> SNADHHAWHRLLDRALSEQHFQLYFQPVVAARDTHLVLHYKVLSRLLDEQGQTIPA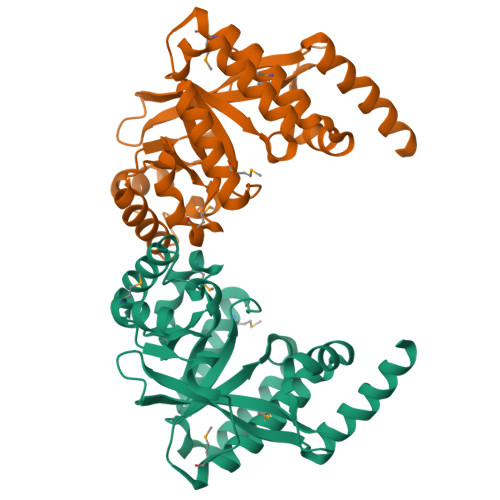GRFLPWLERFGWTSRLDLLMLEQVLRQMASHEDCLALNLSAATLADPHALNRVFEILRQHSDLGPRLTLEIGEEQLPEQAMLEQLTRRLRELGFSLSLQRFGGRFSMIGNLARLGLAYLKIDGSYIRDIDQESDKRLFIEAIQRAAHSIDLPLIAERVETEGELQVIREMGLYGVQGQLFGEPAPWG> GAMANLRTYRA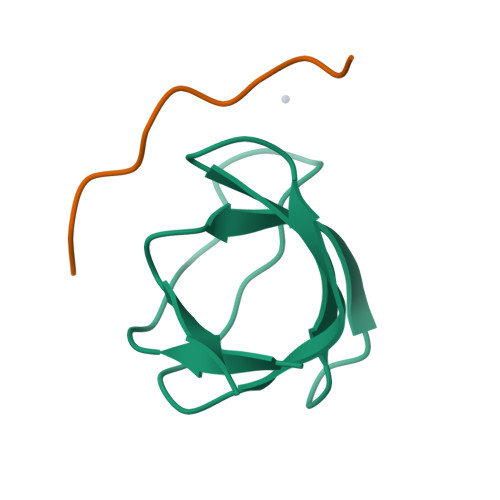MYDYSAQDEDEVSFRDGDYIVNVQPIDDGWMYGTVQRTGRTGMLPANYIEFVN;> PPPTLPKPKLPKH>[2x]MVKLTPELINQSMQYINPVRERELDLRGYKIPQIENLGATLDQFDTIDLSDNDLRKLDNLPHLPRLKTLLLNNNRILRISEGLEEAVPNLGSIILTGNNLQELSDLEPLVGFTKLETISLLINPVSTKPNYREYMAYKFPQLRLLDFRKIKQKDRQAAQEFFRTKQGKDVLKEISR;>[2x]GAMEMLPNQTIYINNLNEKIKKEELKKSLYAIFSQFGQILDIVALKTLKMRGQAFVIFKEIGSASNALRTMQGFPFYDKPMQIAYSKSDSDIVAKIKG

The U1A/U2B″/SNF family of RBPs is found in the U1 and/or U2 small nuclear ribonucleoprotein (snRNP) components of the spliceosome. Jawed vertebrates use U1A to bind stem-loop II of U1 snRNA (U1SLII) and U2B″ in conjunction with the leucine-rich repeat (LRR) protein U2A′ to bind SLIV of U2 snRNA (U2SLIV). Both U1A and U2B″ employ an N-terminal RNA recognition motif (RRM) to specifically recognize their RNA targets. Here, we report crystal structures of four states of dSNFRRM1 at 2 Å resolution or better: the free dSNFRRM1 (residues 1–96; dSNF1–96), dSNF1–96–dU1SLII, dU2A′–dSNF1–96, and dU2A′–dSNF1–96–dU2SLIV. Altogether with the characterization of dSNFRRM1 dynamics alone and in complexes by NMR spectroscopy and targeted mutagenesis combined with binding studies, we delineated how the intrinsic dSNFRRM1 RNA-binding capacity and specificity are fine-tuned by networks of intra-molecular interactions that modulate dSNFRRM1 dynamics, and how the auxiliary dU2A′ protein can capitalize on intrinsic dSNFRRM1 flexibility to gear dSNFRRM1 binding specifically to dU2SLIV.

As in the dSNF1–96–dU1SLII complex, the overall structure of dSNF1–96 is not significantly altered in a crystal structure we determined of a ternary dU2A′–dSNF1–96–dU2SLIV RNP. Significant differences in the shear of the loop-closing U6:G17 wobble pair in U2SLIV compared to the C6:G17 Watson-Crick pair in dU1SLII lead to a different orientation of the two stem regions on dSNF1-96. Instead, Lys17 engages in contacts to the major groove side of U6:G17, as well as to G5 of the adjacent base pair of dU2SLIV; note that an equivalent interaction of Lys17 to the C6:G17 pair in dU1SLII is not equally possible. Concomitantly, Arg49 (L3) is displaced from its position next to A7 in dU1SLII and instead contacts the phosphate of G17 in dU2SLIV. G17 is thereby pulled below the first loop nucleotide (A7), preventing dSNF1–96 Leu46 from stacking on the loop-closing base pair as in the dU1SLII complex. G13 of dU2SLIV adopts a syn conformation to occupy an equivalent position as C13 of dU1SLII, sandwiched by A12 and Asp89 (α3) of dSNF1-96 and hydrogen bonding to the backbone amide of Asp89. U14 adopts the same position in both copies of the ternary complex, resembling the minor conformation of the equivalent C14 of the dSNF1–96–dU1SLII complex, with the base occupying a binding pocket on dSNF1–96. U14 of dU2SLIV can engage in more complementary interactions than a cytidine at the equivalent position, with its Watson-Crick hydrogen bonding potential fully saturated by contacts to Lys20, Lys24 (α1) and the backbone carbonyl of Ala42 (L3). In addition, U14 is held in its position on dSNF1–96 by Arg20 from the N-terminal pincer loop of dU2A′, acting like a lid. Whereas the equivalent U15 and C16 of dU1SLII do not contact dSNF1–96, the additional nucleotide in dU2SLIV allows this RNA region to approach dSNF1–96 more closely, so that Lys20 (α1) can directly contact the phosphates of C15 and C16.>[2x]GMCVEKTPWELVIDFHGHTCPDIALGYRIAQLAQREMGIRPAPDSECLVKAYTQSCALDAIQVLNKATIGRHALIIEETHRYMYQFHFTGTQDIHQFTVSPAVLDHLETLRHPDLSPRERQNKVLEGVQYVLTLEESAFCHYDKIPGQLSKIV

Here, the first crystal structures from PF02663 are described, representing two bacterial and one archaeal species: B8FYU2_DESHY from the anaerobic dehalogenating bacterium Desulfito­bacterium hafniense DCB-2, Q2LQ23_SYNAS from the syntrophic bacterium Syntrophus aciditrophicus SB and Q9HJ63_THEAC from the thermoacidophilic archaeon Thermoplasma acidophilum. Two of these proteins, Q9HJ63_THEAC and Q2LQ23_SYNAS, contain two domains: an N-terminal thioredoxin-like α+β core domain (NTD) consisting of a five-stranded, mixed β-sheet flanked by several α-helices and a C-terminal zinc-finger domain (CTD). The proximity of fmdE to genes encoding the catalytic subunits suggests a role in methanogenesis for proteins in PF02663. Individual proteins within this family display differences in domain architectures, metal-ion binding propensities and dimer interactions.

B8FYU2_DESHY, on the other hand, is composed solely of the NTD. The final model includes two protein molecules (residues 3–151 for chain A; residues 4–151 for chain B), 18 ethylene glycol molecules, one Zn atom, one Ni atom and 427 water molecules in the asymmetric unit. The total β-­sheet and α-helical contents are 24% and 58%, respectively. The monomer consists of a central five-stranded, mixed β-sheet (21345 topology) with one solvent-exposed face, while the other is covered by three α-­helices. A distinctive feature of the structure is the protrusion of two helices (α4 and α5) and a connecting loop (residues 99–138) from the core of each molecule. X-ray anomalous scattering measurements indicated that the site had a mixed occupancy of zinc and nickel. The total occupancy of the zinc and nickel cations was reduced to 0.75 to match the observed scattering at this site, with a zinc:nickel ion stoichiometric ratio of 2.6:1 estimated from the ratio of their anomalous difference map peak heights. Pairwise structural comparisons of B8FYU2_DESHY, Q9HJ63_THEAC and Q2LQ23_SYNAS revealed that the NTDs of B8FYU2_DESHY and Q9HJ63_THEAC are the most similar. The second motif contains Asp58, Gln61 and Thr67 (B8FYU2_DESHY num­bering) and is located along the twofold-symmetry axis at the dimer interface. The absence of a zinc-finger domain in some PF02663 homologs, such as B8FYU2_DESHY, provides some evidence for involvement in alternate processes.> MGKTYYMDPEGSDSNPGTSDKPFATLVKVQEVV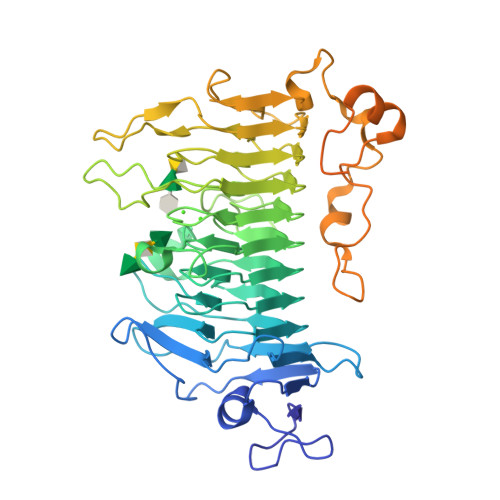VAGDVVYINPGTYVVPANQVPMTTTNSGLYHCVFHMNKSGEAGKPISYLANPNKQGRPIFDLSQVKPKDQRITVFYVTGSNLYLKGFDVIGTQVTITGHTQSECFRIVKGANNNKFEDLRTHDGMAIGFYLLGGSNNHILNCDAYNNYDSVSEGGKGGNVDGFGGHINSSSVGEGKGTGNVFEGCRAWYNSDDGFDLINCFEAVKIINCWSFLNGYKPGTKEVAGDGTGFKAGGYGMAADKLPAIPSVIPQHEVRNSLAYYNRLRGFYANHHLGGIIFESNTAVNSGENYNMTNRESPLALPPTDVNGYDHMVKNNLSLVTRSGSKHIVMVNRAKSEVSNNSFDGSEEVIETDFISLEEAELMRDRKPNGDLPDVNFGKLTTDAELRFWGMGCFATGEPTDLDFGWLKKPTIVVVGSKASVVGPEAASFTKMYVIVDGEETTEFDKNSIDLSDFSGVLEVKAVIEDANGNITKSIALKFKRLEHHHHHH> MTVTRRHFLKLSAGAAVAGAFTGLGLSLAPTVARAELQKLQWAKQTTSICCYCAVGCGLIVHTAKDGQGRAVNVEGDPDHPINEGSLCPKGASIFQLGENDQRGTQPLYRAPFSDTWKPVTWDFALTEIAKRIKKTRDASFTEKNAAGDLVNRTEAIASFGSAAMDNEECWAYGNILRSLGLVYIEHQARIUHSPTVPALAESFGRGAMTNHWNDLANSDCILIMGSNAAENHPIAFKWVLRAKDKGATLIHVDPRFTRTSARCDVYAPIRSGADIPFLGGLIKYILDNKLYFTDYVREYTNASLIVGEKFSFKDGLFSGYDAANKKYDKSMWAFELDANGVPKRDPALKHPRCVINLLKKHYERYNLDKVAAITGTSKEQLQQVYKAYAATGKPDKAGTIMYAMGWTQHSVGVQNIRAMAMIQLLLGNIGVAGGGVNALRGESNVQGSTDQGLLAHIWPGYNPVPNSKAATLELYNAATPQSKDPMSVNWWQNRPKYVASYLKALYPDEEPAAAYDYLPRIDAGRKLTDYFWLNIFEKMDKGEFKGLFAWGMNPACGGANANKNRKAMGKLEWLVNVNLFENETSSFWKGPGMNPAEIGTEVFFLPCCVSIEKEGSVANSGRWMQWRYRGPKPYAETKPDGDIMLDMFKKVRELYAKEGGAYPAPIAKLNIADWEEHNEFSPTKVAKLMNGYFLKDTEVGGKQFKKGQQVPSFAFLTADGSTCSGNWLHAGSFTDAGNLMARRDKTQTPEQARIGLFPNWSFCWPVNRRILYNRASVDKTGKPWNPAKAVIEWKDGKWVGDVVDGGGDPGTKHPFIMQTHGFGALYGPGREEGPFPEHYEPLECPVSKNPFSKQLHNPVAFQIEGEKKAVCDPRYPFIGTTYRVTEHWQTGLMTRRCAWLVEAEPQIFCEISKELAKLRGIGNGDTVKVSSLRGALEAVAIVTERIRPFKIEGVDVHMVGLPWHYGWMVPKNGGDTANLLTPSAGDPNTGIPETKAFMVDVRKVWSHP;> MGKMFFVDLSRCTACRGCQIACKQWKNLPAEETRNTGSHQNPPDLSYVTLKTVRFTEKSRKGPGIDWLFFPEQCRHCVEPPCKGQADVDLEGAVVKDETTGAVLFTELTAKVDGESVRSACPYDIPRIDPVTKRLSKCDMCNDRVQNGLLPACVKTCPTGTMNFGDEQEMLALAEKRLAEVKKTYPGAVLGDPNDVRVVYLFTRDPKDFYEHAVADLAPSMMTRQQLFARLFRPRA

Metal-dependent formate dehydrogenases are important enzymes due to their activity of CO2 reduction to formate. The tungsten-containing FdhAB formate dehydrogenase from Desulfovibrio vulgaris Hildenborough is a good example displaying high activity, simple composition, and a notable structural and catalytic robustness. In these FDHs, the active site is well conserved with the metal being coordinated by four sulfur atoms from two molybdopterin guanosine dinucleotide (MGD) ligands, one labile sulfur and either a S from cysteine or a Se from selenocysteine. FdhAB has the great advantage of being tolerant to oxygen exposure in the oxidized state, allowing its purification and handling in air.

Crystals of the as-isolated enzyme were soaked with dithionite inside an anaerobic chamber, mimicking the conditions of the EPR titration. The resulting crystals (DvFdhAB_dith, PDBcode7Z5O) diffracted beyond 1.5 Å, and the structure was solved by molecular replacement using the formate-reduced structure (PDBcode6SDV). The model was refined to final crystallographic Rwork and Rfree values of 12.1 and 15.3%, respectively. The overall refined structure is identical to that previously determined from crystals soaked with formate, with RMSDs of 0.21 Å for 963 α-carbons (out of 978) in the catalytic subunit and 0.25 Å for 214 α-carbons (out of 236) in the small subunit. On the other hand, in both the dithionite- and formate-reduced structures, the distal MGD-2, which is believed to modulate the redox behavior of the W, suffers a distortion in the ribose moiety, when compared with the as-isolated form. Consistently, the MGD-2 conformational change is thought to be triggered by the rotamer orientation of the Gln890 side chain in the reduced state. Furthermore, analogous to formate, dithionite reduction leads to a small movement of SeCys and its corresponding loop, with Cα-SeCys192 shifting up about 1 Å and the His193 side chain moving away from the metal and being replaced by a water molecule. The adjacent α-helix (Ser194-Pro198) is also displaced up to 2.3 Å (measured at Cα-Thr196). Similar to the formate-reduced form, the catalytic metal site was refined with an occupancy of 1 and very reasonable B-factors (W = 14.9 Å2, S12/1101 = 15.0 Å2, S13/1101 = 15.6 Å2, S12/1102 = 15.1 Å2, S13/1102 = 15.1 Å2, Se = 18.9 Å2, and S = 17.5 Å2). Overall, this structure is nearly identical to the formate-reduced one previously reported, which confirms full reduction by formate.> EVVSLTQAMISQYPAWSVGRSNLQALAGKTCGLAEDVLVELDPNAGMLAPVTAPLADALGAGLSEAFTPNGIPADVTADPVMERPGDRSFLNDDGLITGSEPGTEGGTTAAPGINGSRARLPYNLDPARTPVLGSWRAGVQVPAMLRSGWYRLPTNEQRDRAPLLVVTAAGRFDSREVRLQWATDEQAAAGHHGGSMEFADVGAAPAWRNLRAPLSAIPSTATQVRLVADDQDLAPQHWIALTPPRIPRVRTLQNVVGAADPVFLDWLVGLAFPCQRPFGHQYGVDETPKWRILPDRFGAEANSPVMDHNGGGPLGITELLMRATTVASYLKDDWFRDWGALQRLTPYYPDAQPADLNLGTVTRSGLWSPAPLRRGAPPPPPLGRDPNSSSVDKLAAALEHHHHHH

As a first step towards the complete structural characterisation of the Emb Araf-transferases in M. tuberculosis, we have determined the crystal structure of the hydrophilic C-terminal domain of EmbC, the enzyme responsible for arabinan chain elongation in LAM synthesis and a target for the front line antibiotic EMB. The Emb enzymes of M. tuberculosis display a common architecture of 13 transmembrane helices in conjunction with a hydrophilic C-terminal domain, and share the same polyprenyl donor-substrate, β-D-arabinofuranosyl-1-monophosphoryldecaprenol (DPA). We found that the architecture of this domain comprises two subdomains, one of which folds as a lectin- or CBM-like domain, the other one shows weak similarity to the C-terminal hydrophilic domain of an unrelated GT-C glycosyltransferase, oligosaccharyl transferase STT3. The presence of a CBM-like subdomain in EmbCCT is consistent the proposed role of the C-terminal domain in acceptor substrate recognition.

EmbCCT crystallised in space group P6522 over a diverse range of reservoir conditions, with one molecule in the crystallographic asymmetric unit. EmbCCT is composed of two distinct subdomains, separated by a deep crevice marked by the disordered loops (residues 795–824 and 1016–1037). A high-density peak (14σ, anomalous density difference map) is embedded between loops S3–S4 and S10–S11. Quasi-octahedral coordination geometry and the distribution of peak-ligand distances from 2.40 to 2.63 Å suggest a bound Ca2+ ion. Soaking EmbCCT crystals in cryoprotectant solution containing 27 mM Ara(1→5)Ara-O-C8 (∼3-fold excess of ligand relative to protein concentration in the crystal) reproducibly resulted in defined ligand density, allowing us to unequivocally build one Araf unit and the octyl chain of Ara(1→5)Ara-O-C8, while the second Araf ring remained invisible, even when contouring the map at near-noise level. The soaked di-arabinofuranoside ligand is positioned between two symmetry-related copies of EmbCCT, forming non-covalent contacts only with residues in subdomain I, but not with the CBM-like subdomain II, in contrast to our expectation. The Araf moiety packs against helix H6 and the H6-S13 loop, forming three direct H-bond contacts with protein: O2 binds to carbonyl O of Trp985 (2.53 Å), O1 to Nε1 of Trp985 (2.99 Å), and O3 to Nδ2 of Asn740′ (primed residues indicating the symmetry mate). In contrast, the octyl chain binds between helix H0 and the S13–S14 loop of the symmetry mate. Ligand binding promotes ordering of the N-terminus of helix H0, where 3 additional residues become visible compared to apo, and induces a conformational shift of aspartate residues 1051 and 1052 in the S13–S14 loop. While this crystallographic complex structure did not reveal binding to the CBM-like subdomain II, it is possible that crystal lattice formation of EmbCCT interferes with binding at a site on subdomain II.> GSVTSANLDHTKPCWYWDKKDLAHTPSQLEGLDPATEARYRREGARFIFDVGTRLGLHYDTLATGIIYFHRFYMFHSFKQFPRYVTG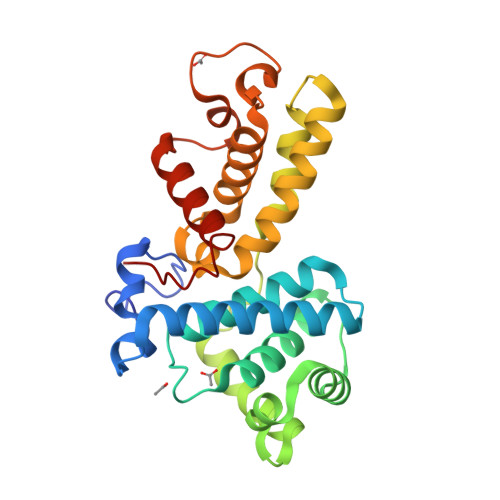ACCLFLAGKVEETPKKCKDIIKTARSLLNDVQFGQFGDDPKEEVMVLERILLQTIKFDLQVEHPYQFLLKYAKQLKGDKNKIQKLVQMAWTFVNDSLCTTLSLQWEPEIIAVAVMYLAGRLCKFEIQEWTSKPMYRRWWEQFVQDVPVDVLEDICHQILDLYSQGKQQMPH>[2x]MGSSHHHHHHSSENLYFQGGGHMTKNSSLLAEFPTCPRDEKDRPRVFTAASGAWLTDESGFRWIDFDNARGSILLGHGDPVVAEAVARAATGADGTATGWSRRVDAVLERLHALCGGEVVGLFRSGTAAVRAAVLAVREATGRPLLLSAGYHGYDPMWYPSEAPLEPNADGVVDFFFDLGLLRELL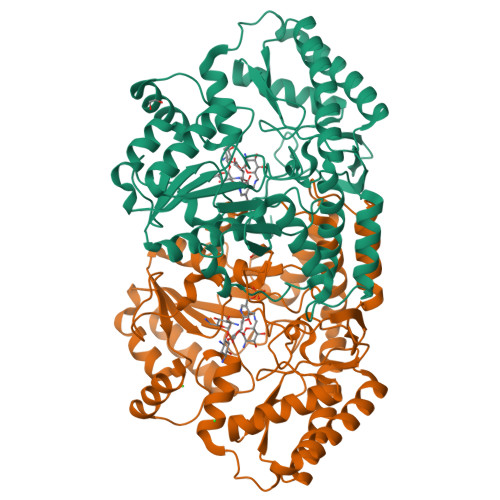RAPERVAAVVVSPDHMHLSPGWYRELRRLCSAAGVVLVADEVKVGLRYAPGLSTAELLAPDVWVVAKGMANGHAVSAVGGSRRLLKPLKEVSFTSFFEPTILAAADAALARVATGEPQRAVREAGDRFLRHARKALDDASLPVEIAGDGTFFQFVPATEELEEALYGAANAEGLLFYAGDNQGVSAAFDEAVLGEAERRFARVCERLAPYAGGEPVGDAARYRVAWNVMDGLRQAPRDREETTGLLARLLDD>[2x]AAIDSTSSSNGSDHHGSSFQAECESFKAKINVTNANVHSVTYVPAGVNISMADNPSICGGDEDPITSTFAFCRIALNVTTSSKSQIFMEAWLPSNYSGRFLSTGNGGLGGCVKYDDMAYAAGYGFATVGTNNGHFGNNGVSFYQNTEVVEDFAYRALHTGVVVGKELTKNFYPQGYNKSYYLGCSTGGRQGWKSVQTFPDDFDGVVAGAPAFNFINLTSWGARFLTLTGDSSAETFVTETQWTAVHNEIIRQCDSLDGAKDGIIEDPDLCQPIIEALLCNATQSSTSGTCLTGAQVKTVNGVFSATYGLNGSFLYPRMQPGSELAAYSSYYSGTPFAYAEDW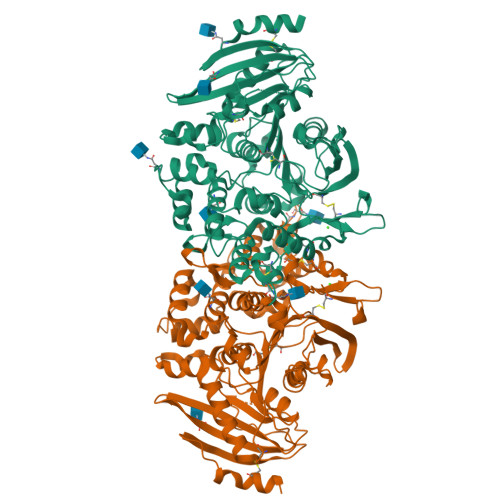YRYVVFNNTNWDVATWTVQDAAIANAQDPYQISTWNGDLSPFQKKGGKVLHYHGMEDAIISSESSKVYYKHVADTMNLSPSELDSFYRFFPISGMAHCANADGPSAIGQGTGTFAGNNPQDNVLLAMVQWVEEGVAPDFVRGAKLNGSTVEYRRKHCKYPKRNRYVGPGSYTDENAWECV>GSHMKLCLVCSDEASGCHYGVLTCGSCKVFFKRAVEGQHNYLCAGR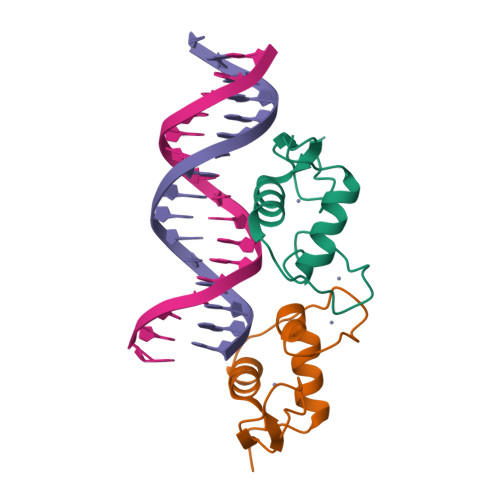NDCIIDKIRRKNCPACRYRKCLQAGMNLEARKTKKKIKGIQQATT[2x]>[4x]GSKESPLHGTQNTINKRTQPTFGFTVNWKFSESTTVFTGQCFIDRNGKEVLKTMWLLRSSVNDIGDDWKATRVGIMIFTRLRTQKEGGSGGSARKCSLTGKWTNDLGSNMTI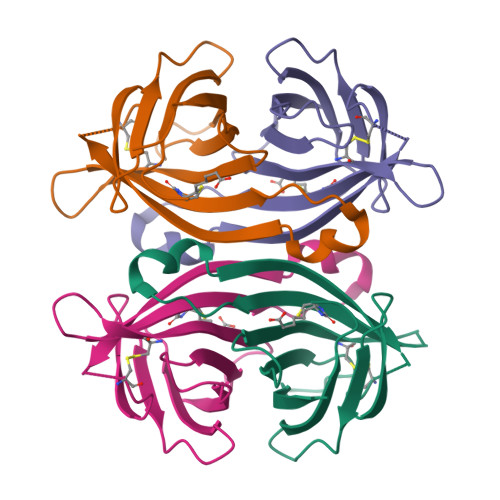GAVNSRGEFTGTYITAVT>MEQEKVQELVSQMTLDEKIAQCLQLSPFLFKGTNKNAELTGPLLQEMKLTDAHTENAGSVLGSSSALDMIGIQEAYLKTNRLGIPLVFMADVIHGYKTVFPIPLALGCSFDRETVRVMAEVSALEATADGHHVTFSPMLDLVRDPRWGRVMESTGEDPFLNSELGKAMVDGYQGDASKLNENLEQMAACVKHFAAYGAAEAGLEYNTVNMSTRELYQNYLPAYNAAIQAGAKLVMTAFNVVDGIPATMNKWLNRDVLRGEMEFDGVLISAWGAVAEVINHGTARNPKEAAQFSMEAGVDLEMMTTCYIHELKGLIEEGKLSENLLDEAVLRMLNLKNDLGLFEDPYRGLKNNDRTKDILTDESRGKARAAGVESAVLLENKSRLLPLAKEAKIALVGPLATSPDILGGWNVYGEEKDGINVETGLREVFETVEVVSTEYTELSEEDKVAVKAAVQNMDVVVLALGEKNEWGGEAGSLATIRLPEAQYQLAKFVQTLGKPVVITLFNGRPLEVKELAESSDALLELWFPGTEAGRVTADLLSGASNPSGKLSMSFPQTTGQIPVYYNHLRTGRPQTPENKGERYVSHYLDIPNEPFYPFGYGKSYSEFELKTSSLPKELNLGESLHVEVTIKNISDIAGKEVIQVYLQDVTASISRPVKELKAFEKV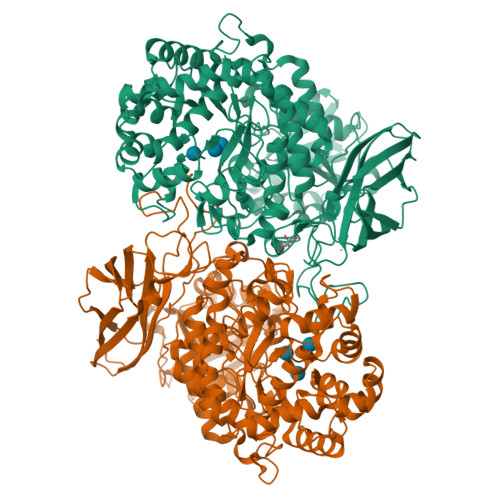ALQAGEEKTVTFELTSEAFSFYNHQLEKVQEPGLHRVFVGTSSEDVDVFEVEVGGYVLEHHHHHH[2x]> NLFQFGDMILQKTGKEAVHSYAIYGCYCGWGGQGRAQDATDRCCFAQDCCYGRVNDCNPKTATYTYSRENGDIV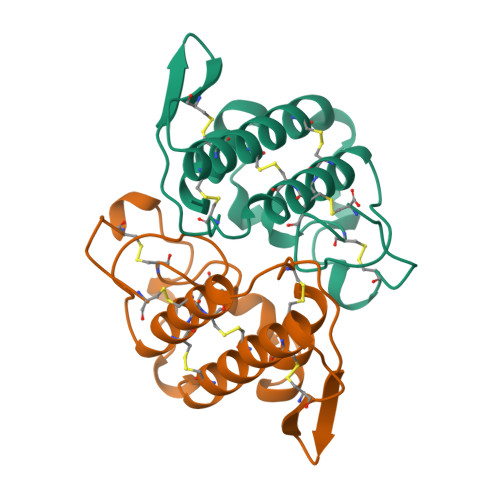CGDDDLCLRAVCECDRAAAICLGENVNTYDKNYEYYSISHCTEESEQC;> NLFQFAKMINGKLGAFSVWNYISYGCYCGWGGQGTPKDATDRCCFVHDCCYGRVRGCNPKLAIYYYSFKKGNIVCGKNNGCLRDICECDRVAANCFHQNKNTYNANYKFLSSSRCRQTGEKC>[2x]MAHHHHHHMTRVLAVANQKGGVAKTTTVASIGAALTEQGRRVLLVDLDPQGCLTFSLGHDPDKLPVSVHEVLLGDVEPSAALVRTDEGMTLLPANIDLAGAEAMLLMRAGREYALKRALAKLDGDFDVVIIDCPPSLGVLTLNGL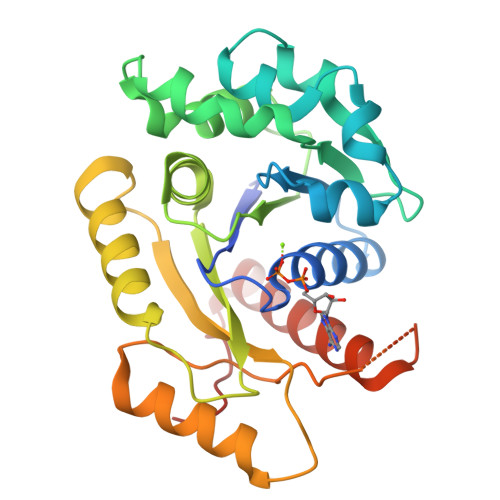TAAHDVIVPLQCETLAHRGVGQFLRTISDVQQITNPDLKLLGALPTLYDSRTTHSRDVLLDVADRYELPVLAPPIPRTVRFAEASASGSSVLAGRKSKGAIAYREFADALLRHWKSGRKMPTFTPEVV> MPVLLGI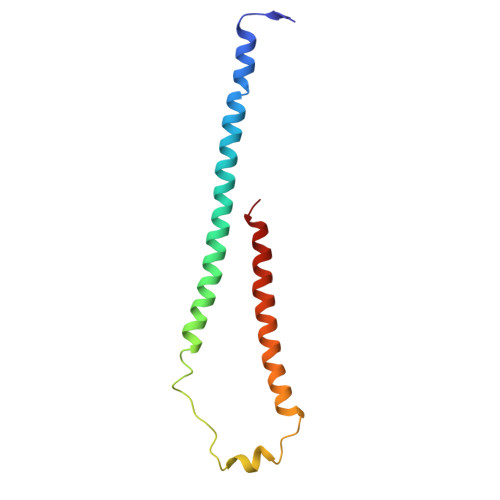PLLLRFLGFLLVTLFGYLLTFLKKGFGKIAIAISLFLALIIGLNSILVGYLSDISAQLPSDFVQGVQLILPSNALPCFYVILSVKAAIFIFDVKQKIVSYLDWDK(2R)-3-{[4-(4-chloro-3-ethylphenoxy)pyrimidin-2-yl][3-(1,1,2,2-tetrafluoroethoxy)benzyl]amino}-1,1,1-trifluoropropan-2-ol 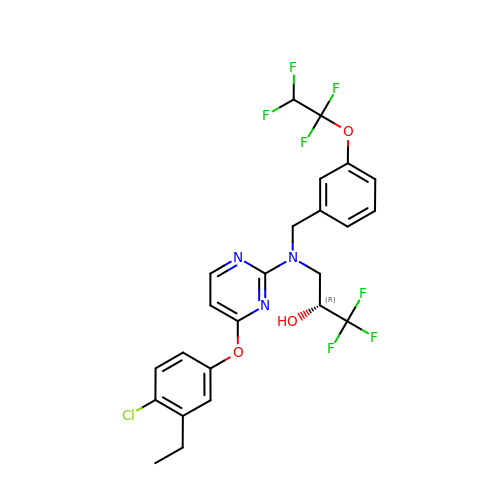| C24 H21 Cl F7 N3 O3 | BTIIJGFMCVLCET-LJQANCHMSA-N> ALMGGIVDVEGAQNSAEVEELARFAVDEHNKKENA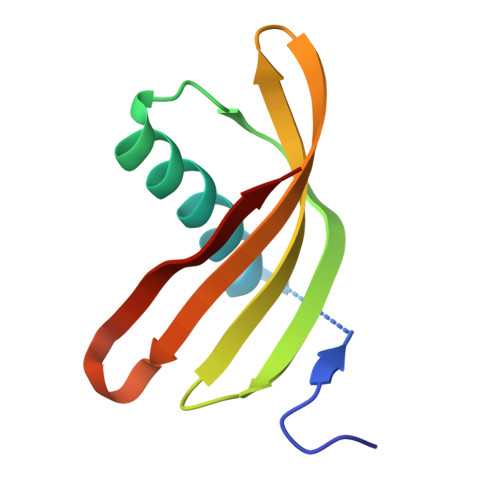LLQFSRLVKAKQQVVSGIMHHLTVEVIEGGKKKVYEAKVWVQAWLNSKKLHEFSPI> MHHHHHHHHHHGENLYFQGSDNIISFDHVTFTYPDSPRPALSDLSFAIERGSWTALIGHNGSGKSTVSKLINGLLAPDDLDKSSITVDGVKLGADTVWEVREKVGIV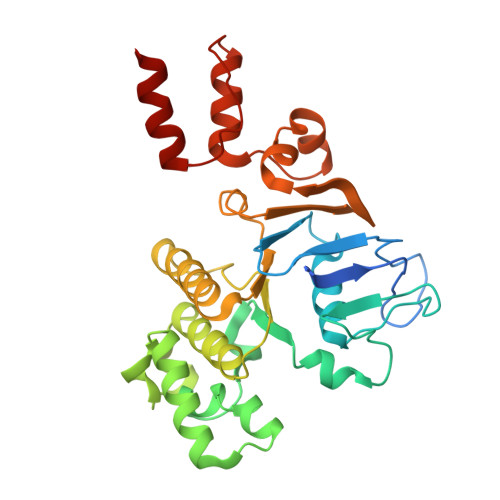FQNPDNQFVGATVSDDVAFGLENRAVPRPEMLKIVAQAVADVGMADYADSEPSNLSGGQKQRVAIAGILAVKPQVIILDESTSMLDPEGKEQILDLVRKIKEDNNLTVISITHDLEEAAGADQVLVLDDGQLLDQGKPEEIFPKVEMLKRIGLDIPFVYRLKQLLKERGIVLPDEIDDDEKLVQSLWQLNS The membrane-anchored SNARE (soluble N-ethylmaleimide-sensitive factor acceptor protein receptor) proteins provide the energy to drive membrane fusion in various cellular contexts, such as intracellular trafficking and exocytosis. Supercomplexes of NSF, α-SNAP, and either a syntaxin tetramer or one of two binary complexes of syntaxin—SNAP-25 reveal atomic details of SNARE processing and show how sequential ATP hydrolysis drives disassembly. NSF comprises three structured domains connected by flexible linkers—the adapter N-domain followed by the D1 and D2 AAA+ domains. Six NSF protomers come together to form the active form of the enzyme, a homo-hexamer.

To gain insight into the structural nature of binary complex formation and disassembly by NSF, we prepared a complex of NSF, ɑ-SNAP, and the binary t-SNARE complex (21bin20S) composed of full-length soluble SNAP-25 and soluble syntaxin-1a (1–267) in the absence of divalent cation (i.e., non-hydrolyzing conditions) and performed single-particle cryo-EM. Classes with evidence of NSF D1 domains engaging ordered ɑ-SNAP—SNARE sub-complexes were carried forward; eight 21bin20S models were built into reconstructions ranging from 3.39–4.01 Å in resolution, differing mainly in the orientation of N domains and a sub-complex of three ɑ-SNAP molecules and four SNARE motifs relative to the D1 ATPase ring. All classes revealed substrate-bound NSF without Mg2+ needed for ATP hydrolysis and disassembly, and share the same overall architecture, with a spire composed of NSF N-domains and the ɑ-SNAP—SNARE subcomplex on top, the NSF D1 ring in the middle tier, and the NSF D2 ring forming the bottom tier. A representative 21bin20S model (class #5, 3.39 Å) and ɑ-SNAP—2:1 binary SNARE subcomplex model (class #13, 3.74 Å). A Hexameric NSF engages the ɑ-SNAP—2:1 binary SNARE subcomplex via multiple N-domains (salmon), which engage three ɑ-SNAP molecules (gold) surrounding the 2:1 binary SNARE complex composed of two syntaxin H3 domains (dark red) and the SN1 and SN2 SNARE domains of a single SNAP-25 molecule (green). A linker N-terminal to one of the syntaxin H3 domains is found within the catalytic D1 ring of NSF (light blue). The D2 ring of NSF (purple) does not engage substrate. B NSF (light blue) engages one of the two syntaxin molecules in the 2:1 binary SNARE complex (dark red) via pore loop interactions involving Y294 (protomers A–F, indicated). Three ɑ-SNAP molecules bind the 2:1 binary SNARE complex; a flexible linker between SNAP-25 SN1 and SN2 blocks access by a fourth. Of the eight 21bin20S classes with the 2:1 binary SNARE complex from the dataset collected under non-hydrolyzing conditions, six engage syntaxin and two engage SNAP-25 within the pore of the D1 ring.

>[6x]GAHMAGRSMQAARCPTDELSLSNCAVVSEKDYQSGQHVIVRTSPNHKYIFTLRTHPSVVPGSVAFSLPQRKWAGLSIGQEIEVALYSFDKAKQCIGTMTIEIDFLQKKNIDSNPYDTDKMAAEFIQQFNNQAFSVGQQLVFSFNDKLFGLLVKDIEAMDPSILKGEPASGKRQKIEVGLVVGNSQVAFEKAENSSLNLIGKAKTKENRQSIINPDWNFEKMGIGGLDKEFSDIFRRAFASRVFPPEIVEQMGCKHVKGILLYGPPGCGKTLLARQIGKMLNAREPKVVNGPEILNKYVGESEANIRKLFADAEEEQRRLGANSGLHIIIFDEIDAICKQRGSMAGSTGVHDTVVNQLLSKIDGVEQLNNILVIGMTNRPDLIDEALLRPGRLEVKMEIGLPDEKGRLQILHIHTARMRGHQLLSADVDIKELAVETKNFSGAELEGLVRAAQSTAMNRHIKASTKVEVDMEKAESLQVTRGDFLASLENDIKPAFGTNQEDYASYIMNGIIKWGDPVTRVLDDGELLVQQTKNSDRTPLVSVLLEGPPHSGKTALAAKIAEESNFPFIKICSPDKMIGFSETAKCQAMKKIFDDAYKSQLSCVVVDDIERLLDYVPIGPRFSNLVLQALLVLLKKAPPQGRKLLIIGTTSRKDVLQEMEMLNAFSTTIHVPNIATGEQLLEALELLGNFKDKERTTIAQQVKGKKVWIGIKKLLMLIEMSLQMDPEYRVRKFLALLREEGASPLDFD;>[2x]MKDRTQELRTAKDSDDDDDVTVTVDRDRFMDEFFEQVEEIRGFIDKIAENVEEVKRKHSAILASPNPDEKTKEELEELMSDIKKTANKVRSKLKSIEQSIEQEEGLNRSSADLRIRKTQHSTLSRKFVEVMSEYNATQSDYRERCKGRIQRQLEITGRTTTSEELEDMLESGNPAIFASGIIMDSSISKQALSEIETRHSEIIKLENSIRELHDMFMDMAMLVESQGEMIDRIEYNVEHAVDYVERAVSDTKKAVKYQSKARRKKIM;> MGSSHHHHHHSQDPNSMAEDADMRNELEEMQRRADQLADESLESTRRMLQLVEESKDAGIRTLVMLDEQGEQLERIEEGMDQINKDMKEAEKNLTDLGKFAGLAVAPANKLKSSDAYKKAWGNNQDGVVASQPARVVDEREQMAISGGFIRRVTNDARENEMDENLEQVSGIIGNLRHMALDMGNEIDTQNRQIDRIMEKADSNKTRIDEANQRATKMLGSG;>[3x]GMDTSGKQAEAMALLAEAERKVKNSQSFFSGLFGGSSKIEEACEIYARAANMFKMAKNWSAAGNAFCQAAQLHLQLQSKHDAATCFVDAGNAFKKADPQEAINCLMRAIEIYTDMGRFTIAAKHHISIAEIYETELVDVEKAIAHYEQSADYYKGEESNSSANKCLLKVAGYAAQLEQYQKAIDIYEQVGTSAMDSPLLKYSAKDYFFKAALCHFCIDMLNAKLAVQKYEELFPAFSDSRECKLMKKLLEAHEEQNVDSYTESVKEYDSISRLDQWLTTMLLRIKKTIQGDEEDLR> GAMDMSKELLLVVDAVANEKGVPREVIFDAIEAALASAAKKRYPDQDVLARVTIDHKDGTYETYRRWEVVADDVVMESPDRQVRLMDAIDEADGVDVGDYIEEQIENPDFGRIAAQAAKQVIVQRVREAERQQVVDAWKDRVGELITGVVKRAERGNIFVDLGGNAEAFIPKDKGIPRDVLRPGDRVRGYLAEVRSEPRGPQLFISRAAPEFMIELFKLEVPEVGQGLVEINACARDPGD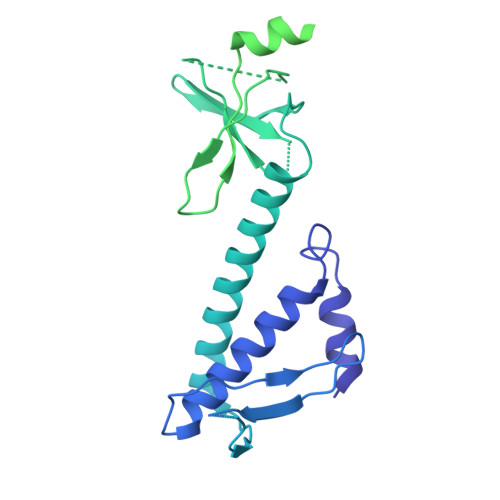RAKIAVIAHDARTDPIGACIGMRGSRVQAVSNELNGERVDIVLWNENPANFVINAMAPAEVQSIIVDEDKHSMDLAVAEDRLAQAIGKGGQNVRLASRLTGWQLNVMTADQVAAKSEAEQAAARQLFMDRLEVDEEISAILVSEGFNTVEEIAYVPVGELLAVEGFDEDIVEELRARARDALLNAALAEEEGLEGTQPTEDLLALEGMDEETAVALAEHGVRTSEDLSDLAADEIVDFGIEGLTQERAAALILAARAEEIARLERGE> MNMSGGGEQADILPANYVVKDRWKVLKKIGGGGFGEIYEAMDLLTRENVALKVESAQQPKQVLKMEVAVLKKLQGKDHVCRFIGCGRNEKFNYVVMQLQGRNLADLRRSQPRGTFTLSTTLRLGKQILESIEAIHSVGFLHRDIKPSNFAMGRLPSTYRKCYMLDFGLARQYTNTTGDVRPPRNVAGFRGTVRYASVNAHKNREMGRHDDLWSLFYMLVEFAVGQLPWRKIKDKEQVGMIKEKYEHRMLLKHMPSEFHLFLDHIASLDYFTKPDYQLIMSVFENSMKERGIAENEAFDWEKAGTDALLS

Tau tubulin kinase 1 and 2 (TTBK1/2) are understudied serine/threonine/tyrosine kinases that belong to the casein kinase 1 superfamily. Their kinase domains have 88% identity, 96% similarity, and the same catalytic residues: lysine 63 and aspartic acid 164 (TTBK1) and lysine 50 and aspartic acid 141 (TTBK2). As their names imply, TTBK1/2 are reported to phosphorylate tubulin and tau at multiple serine residues. We have described the design, synthesis, and biological evaluation of a series of indolyl pyrimidinamines as chemical tools to interrogate the functions of TTBK1/2.

Our lead (AMG28) emerged from examination of the off-target activity of a published Amgen NF-κB inducing kinase (NIK) inhibitor. The potency of AMG28 was reported in the MRC Kinase Profiling Inhibitor Database as 8% activity remaining for TTBK1 and 12% activity remaining for TTBK2 when screened at 1 μM. Biogen evaluated AMG28 in a biochemical assay (TTBK1 IC50 = 199 nM) and a cellular assay that measures inhibition of tau phosphorylation at Ser422 (IC50 = 1.85 μM). The aminopyrimidine ring makes two key hydrogen bonds with TTBK1 backbone hinge residues Q108 and Q110. Except for AMG28, which was equipotent on both kinases, all analogs were more potent inhibitors of TTBK2 than TTBK1. The enzymatic data for this small series supports that the seven-membered ring offers enhanced efficacy versus the smaller and larger ring systems. We propose that the ring system size alters the orientation and trajectory of the alkyne and the ability of the compounds to make key contacts with the back pocket is diminished with analogs 1 and 2 compared to AMG28. All inhibitors, including AMG28, that protrude into the back pocket produce remarkably higher Tm shift values than TTBK inhibitors that are unable to access the back pocket, including those built upon the AZ2 scaffold (ΔTm < 3.5), when tested in parallel.>SAPRPCQAPQQWEGRQVMYQQSSGRNSRALLSYDGLNQRVRVLDERKALIPCKRLFEYILLYKDGVMFQIDQATKQCSKMTLTQPWDPLDIPQNSTFEDQYSIGGPQEQITVQEWSDRKSARSYETWIGIYTVKDCYPVQETFTINYSVILSTRFFDIQLGIKDPSVFTPPSTCQ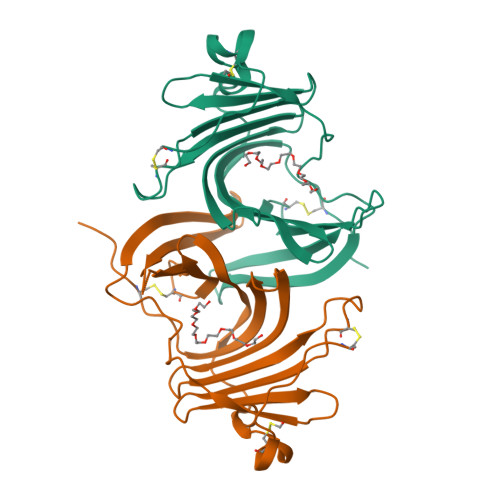MAQLEKMSEDCSWHHHHHH[2x]> SDLIPAPPLSKVPLQQNFQDNQFHGKWYVVGVAGNGFLREDKDPIKMAATIYELKEDKSYNVTFQKFPMKKCQYMTDTLVPGSQPGEFTLGNIKSEPGYTSWLVRVVSTNYNQHAMVFFKAVQQNREDFFITLYGRTKELTSELKENFIRFSKS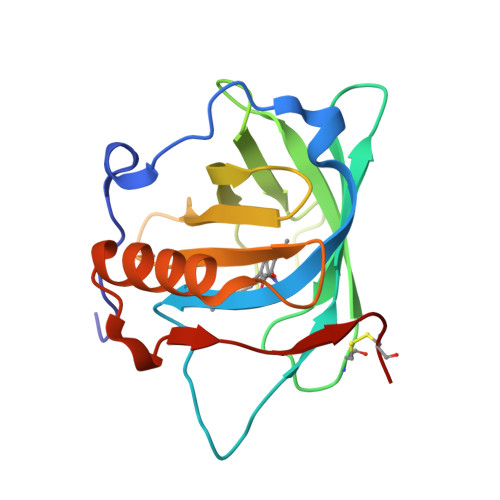LGLPENHIVFPVPIDQCIDG> ISEFMAKIETLEEALKAAEALEREGVHAILDLLGEMVRTEEEARAFQRGLLELVWALAGKPWPKYISLKLTQLGLDLSEDLALALLREVLREAEPRGVFVRLDMEDSPRVEATLRLY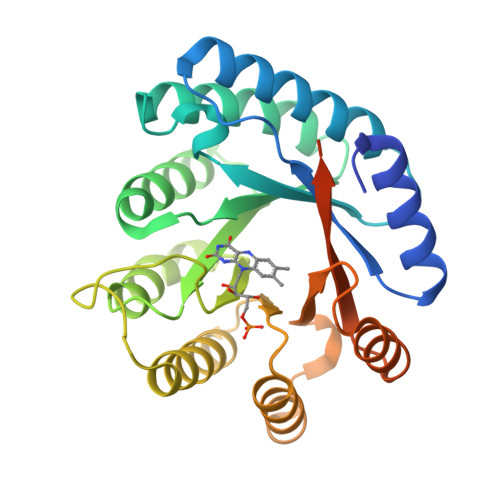RALREEGFSQVGIVLQSYLYRTEKDLLDLLPYRPNLRLVKGAYREPKEVAFPDKRLIDAEYLHLGKLALKEGLYVAFATHDPRIIAELKRYTEAMGIPRSRFEFQFLYGVRPEEQRRLAREGYTVRAYVPYGRDWYPYLTRRIAERPENLLLVLRSLVSGLE> GKAPVDPECTAKVGKAHVYCEGNDVYDVMLNQTNLQFNN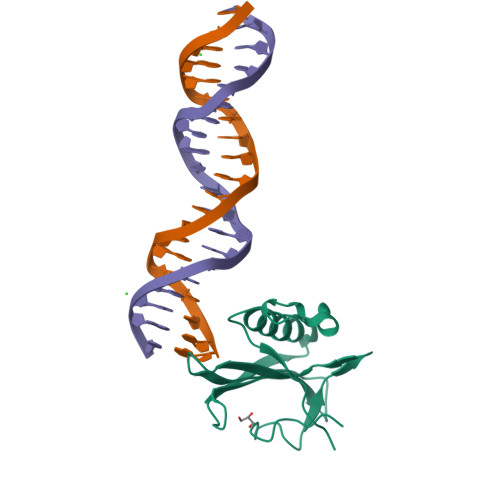NKYYLIQLLEDDAQRNFSVWMRWGRVGKMGQHSLVACSGNLNKAKEIFQKKFLDKTKNNWEDREKFEKVPGKYDMLQMDYATNTQDEEET> MIDLTAFLTLLRA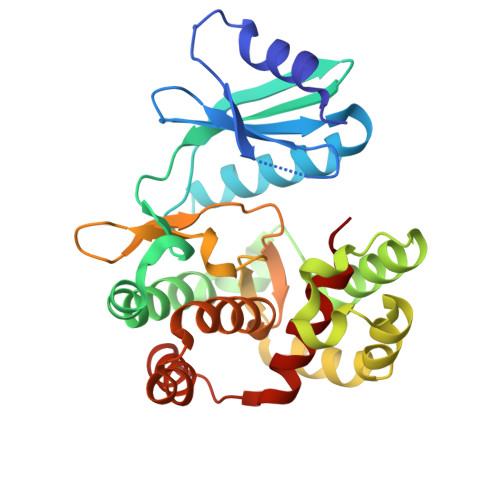DGGDAGWEPVTDGESGAAVFRSADGSRYAKCVPADQVAALEAERDRVSWLSTQDIPGPRVLDWRVGAAGAGLLTSTVEGIPADRASASMLRAAWEPIADAVRRLHELPPEKCPFTRELGEMFSMARDVVAREAVNPDFLPEEQRHTPPGELLARLAPYVGQRLAQEAAQTVVCHGDLCLPNIILDPDTLDVAGFIDLGRLGRADPYADLALLFATARETWGDDERWSQSAEEEFAARYGIALDRDRERFYLHLDPLTWG>[2x]AFGVEPYGQPKYLEIAGKRMAYIDEGKGDAIVFQHGNPTSSYLWRNIMPHLEGLGRLVACDLIGMGASDKLSPSGPDRYSYGEQRDFLFALWDALDLGDHVVLVLHDWGSALGFDWANQHRDRVQGIAFMEAIVTPMTWADWPPAVRGVFQGFRSPQGEPMALEHNIFVERVLPGAILRQLSDEEMNHYRRPFVNGGEDRRPTLSWPRN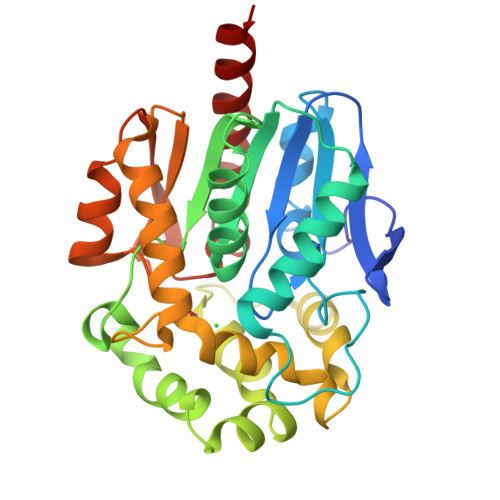LPIDGEPAEVVALVNEYRSWLEETDMPKLFINAEPGAIITGRIRDYVRSWPNQTEITVPGVHFVQEDSPEEIGAAIAQFVRRLRSAAG> MSEAIIAAARGRLISPPFSDATGDVYRTPEAALPAIIVELDYTDAERISMGGGFIASA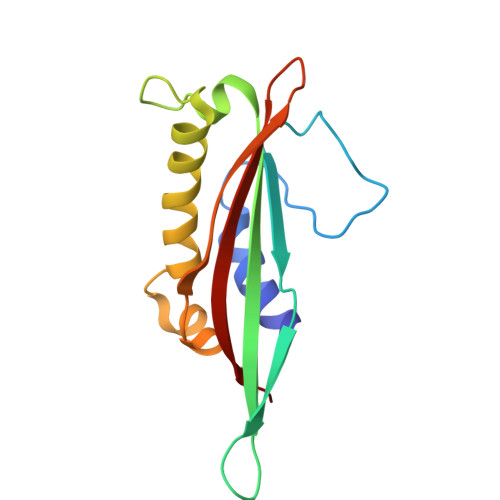ELRVEILAKRDDWSLLTPTPANTAEGMARLAALVRTAILAPPSDLSGLAWSIAPAGYEFETERGETPLARATQSFALQILQP>[6x]MGSDKIHHHHHHMKTDTEWLLCDFHVHTNMSDGHLPLGEVVDLFGKHGVDVVSITDHIVDRRTLEQRKRNGEPLGAITEDKFQDYLKRLWREQKRAWEEYGMILIPGVEITNNTDLYHIVAVDVKEYVDPSLPVEEIVEKLKEQNALVIAAHPDRKK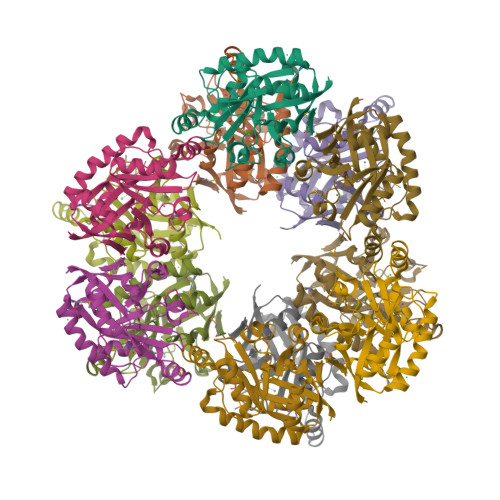QDEEHLSWYLWANMERFKDTFDAWEIANRDDLFNSVGVKKYRYVANSDFHELWHVYSWKTLVKSEKNIEAIKEAIRKNTDVAIYLMRKNRLSSLSDVI> SSGAIIYTVELKRYGGPLGITISGTEEPFDPIIISSLTKGGLAERTGAIHIGDRILAI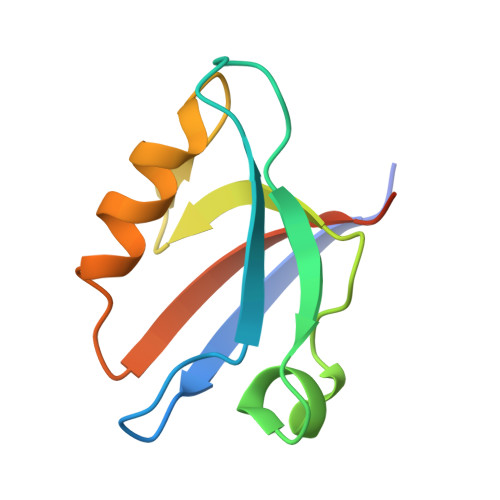NSSSLKGKPLSEAIHLLQMAGETVTLKIKKQTDAQPASS>[2x]VAPLDLVQPISDYKIYVSENLQTLVRDTREFTNAVKAGDVAKAKKLFASTRMSYERIEPIAELFSDLDASIDSRADDHEKAEKDPAFFGFHRIEYGLFAQNSAKGLAPVADKLMADVLELQKRIRGLTFPPEKVVGGAAVLMEEVAATKISGEEDRYSHTDLWDFQANFEGAKKIVDLFRPLVVKDNRAFADKVDANFDTVFKTLAKYRTADGGFELYGKLSERDRKVLA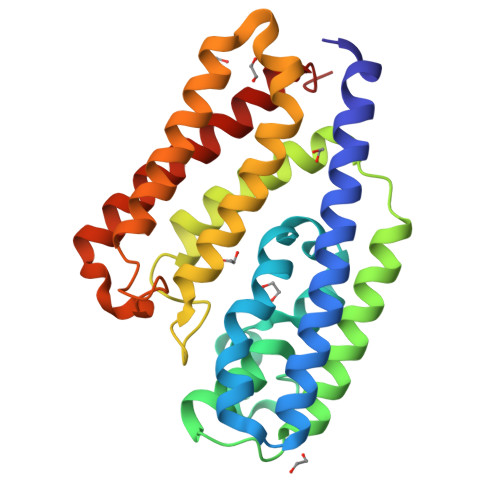GRVNTLAEDLSKMRGLLGLDL The protein, termed Pa Dps, adopts the Dps subunit fold and oligomerizes into a nearly spherical 12-mer quaternary structure at pH 6.0 or in the presence of divalent cations at neutral pH and above. The 12-Mer Pa Dps contains two di-iron centers at the interface of each subunit dimer, coordinated by conserved His, Glu, and Asp residues. In vitro, the di-iron centers catalyze the oxidation of Fe2+ utilizing H2O2 (not O2) as an oxidant, suggesting Pa Dps functions to aid P. aeruginosa to survive H2O2-mediated oxidative stress. The Pa Dps structure harbors a novel network of Tyr residues at the interface of each subunit dimer between the two di-iron centers, which captures radicals generated during Fe2+ oxidation at the ferroxidase centers and forms di-tyrosine linkages, thus effectively trapping the radicals within the Dps shell.

The screening of crystallization conditions produced two crystal forms, prismatic crystals of a primitive orthorhombic form (Dps-o) and primitive cubic lattice crystals (Dps-c). Structure solution and refinement resulted in a Dps-o model containing 12 subunits in the asymmetric unit. One sodium ion and two chloride ions bind to each subunit, and 82 sulfate ions (acquired from the crystallization solution) are associated with the 12-mer. The 12-mer assembly forms a nearly spherical shell (23-point group symmetry, ~9 nm diameter), which surrounds a hollow interior cavity (~4 nm diameter). The Cl− associated with each subunit is surrounded by residues in the long loop and residues in α5. The Na+ is located at inter-subunit sites coordinated by H37 from one subunit and D64 and E68 from the second subunit; only five of the twelve D64 residues coordinate a sodium ion in the structure, and these may be interchangeable with water molecules. The Dps-o structure revealed the presence of a Na+ coordinated by ferroxidase center ligands H37, D64, and E68. Each pair of three-fold pores along a three-fold axis exhibits distinct microenvironments, giving rise to two types of three-fold pores, termed here A and B. In the A-type three-fold pores, residues near the turn separating α1 and α2 form the pore trimeric interface, which is defined by P43, N46, T47, M44, and E100, and in the model contains an SO42−, which forms water-mediated contacts with the backbone N-atom of N46. The electrostatic surface of the A-type three-fold pore interior is positive, which probably stabilizes the SO42− ion, while the electrostatic surface in the immediate vicinity of the pore exterior is negative and is surrounded by three patches of positive potential where the SO42− and Cl− ions in the structure nest. The Dps-c structure is nearly identical to the Dps-o structure, as indicated by the 0.38 Å RMSD deviation observed on superposing the Cα atoms in the dodecamers (1832 residues).

>[12x]MEINIGIGEQDRAAIAEGLSRLLADTYTLYLKTHNFHWNVTGPMFNTLHLMFEGQYTELAVAVDDIAERIRALGFPAPGTYAAYARLSSIKEEEGVPEAEEMIRQLVQGQEAVVRTARSIFPLLDKVSDEPTADLLTQRMQVHEKTAWMLRSLLAS> GSVKRVVYKKRPNLIISNVGY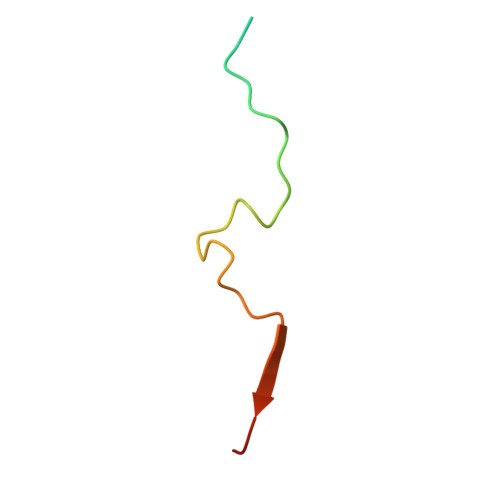SELRKPEGVISGRKTFGDNSD> MADDVDNDDKLEKPVDLIWGCELNEQNKTFEFKVEDDEEKCEHQLALRTVCLGDKAKDEFHIVEIVDQEEGAEKSVPIATLKPSILPMATMVGIELDPPVTFRLKAGSGPLYISGQ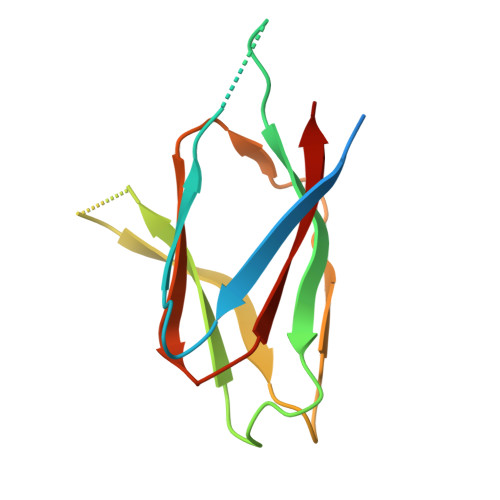HVAM> MPIMLEDYQKNFLELAIECQALRFGSFKLKSGRESPYFFNLGLFNTGKLLSNLATAYAIAIIQSDLKFDVIFGPAYKGIPLAAIVCVKLAEIGGSKFQNIQYAFNRKEAKDHGEGGIIVGSALENKRILIIDDVMTAGTAINEAFEI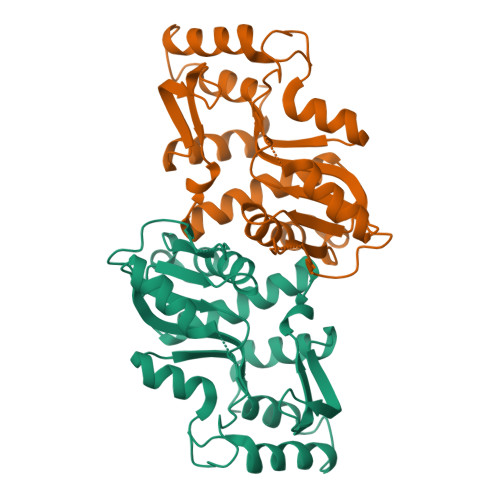ISNAKGQVVGSIIALDRQEVVSTDDKEGLSATQTVSKKYGIPVLSIVSLIHIITYLEGRITAEEKSKIEQYLQTYGASA(2~5~S)-2~3~,2~5~,2~6~-trihydroxy[1~1~,2~1~:2~4~,3~1~-terphenyl]-2~2~(2~5~H)-one 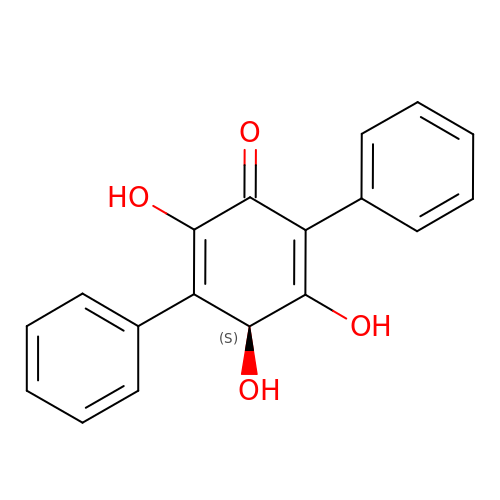| C18 H14 O4 | ODPMSLCGNZJREU-HNNXBMFYSA-N> ASHMKFTVEREHLLKPLQQVSGPLGGRPTLPILGNLLLQV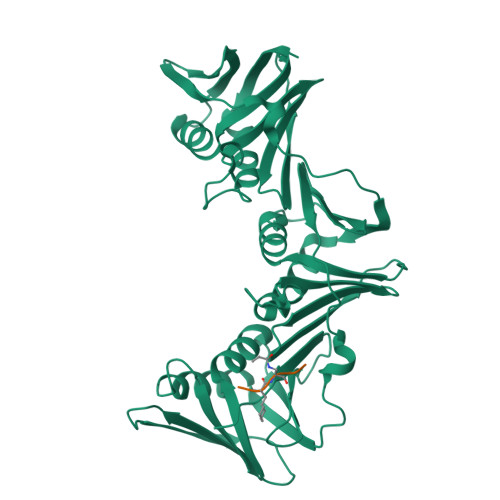ADGTLSLTGTDLEMEMVARVALVQPHEPGATTVPARKFFDICRGLPEGAEIAVQLEGERMLVRSGRSRFSLSTLPAADFPNLDDWQSEVEFTLPQATMKRLIEATQFSMAHQDVRYYLNGMLFETEGEELRTVATDGHRLAVCSMPIGQSLPSHSVIVPRKGVIELMRMLDGGDNPLRVQIGSNNIRAHVGDFIFTSKLVDGRFPDYRRVLPKNPDKHLEAGCDLLKQAFARAAILSNEKFRGVRLWVSENQLKITANNPEQEEAEEILDVTYSGAEMEIGFNVSYVLDVLNALKCENVRMMLTDSVSSVQIEDAASQSAAYVVMPMRL>NNSIIDQNVQALFNEISADAVFVTYDGQNIKKYGTHLDRAKTAYIPASTFKIANALIGLENHKATSTEIFKWDGKPRFFKAWDKDFTLGEAMQASTVPVYQELARRIGPSLMQSELQRIGYGNMQIGTEVDQFWLKGPLTITPIQEVKFVYDLAQGQLPFKPEVQQQVKEMLYVERRGENRLYAKSGWGMAVDPQVGWYVGFVEKA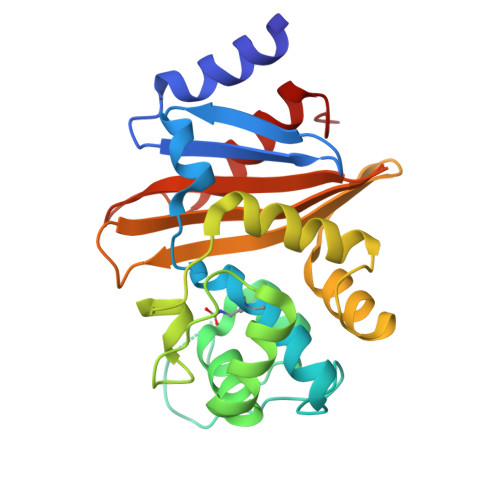DGQVVAFALNMQMKAGDDIALRKQLSLDVLDKLGVFHYL[4x]> MAFLKVVPLEKALEVVQSFKISPG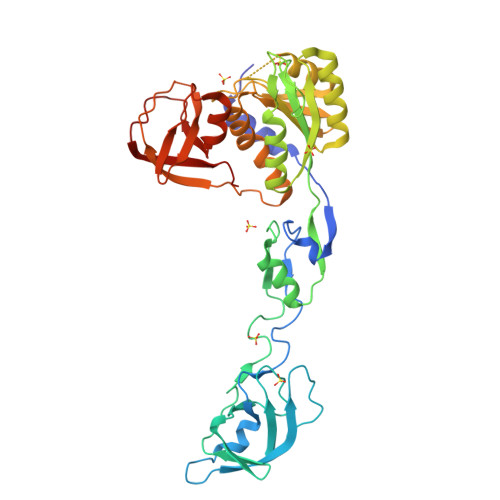IEEVPIEKGLGRIAAEDIYSPIDVPPFDRATVDGYAVRAEDTFMASEASPVRLKVIGSVHAGEEPKFKLGKGEAAYISTGAMLPGNADAVIQFEDVERVNGEILIYKPAYPGLGVMKKGIDIEKGRLLVKKGERLGFKQTALLSAVGINKVKVFRKPKVAVISTGNEIVPPGNELKPGQIYDINGRALCDAINELGGEGIFMGVARDDKESLKALIEKAVNVGDVVVISGGASGGTKDLTASVIEELGEVKVHGIAIQPGKPTIIGVIKGKPVFGLPGYPTSCLTNFTLLVVPLLLRALGREGKIGKKVARLKHKVFSVKGRRQFLPVKLEGDLAVPILKGSGAVTSFIDADGFVEIPETVESLDEGEEVEVTLFKGW> AMELIRIAMKKDLENDNSLMNKWATVAGLKNPNPLYDFLNHDGKTFNEFSSIVNIVKSQYPDREYELMKDYCLNLDVKTKAARSALEYADANMFFEIEDALIDSMISCSNMKSKEYGKVYKIHRELSKGEIDVFEASANIGKQRIKTAEMNIFSKMLLMYDCLNKGNFAPMMLLFQQIDLSEIKENRYLKNSFETRINVLLSNIYLNENNLELCREYAQKAISSTDTQRFLVFSYLTIGTSYIFSDFNLSKQNYLIGLKFAKGNPGFEEFFKRNLSFLNNFWNKENEWINYDSDAVTDMQEVIFELINHKELSKALQLLNKLEERDQNENELGFHYYLKGLITNEKEAFFKSVEYFKASQDKLSIKMPLIQLEK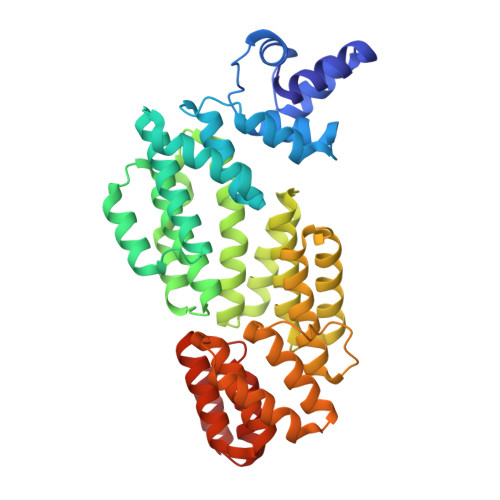MGENPRLLKIITM>GPLGSIYSPHETLAEKHSEKKLMDSFSPSLSQDKMDGEFAHANIDGISIRLCLNKGICSVFYLDGDKIQSTQLSSKEYNNLLSSLPPKQFNLGKVHTITAPVSGNFKTHKPAPEVIETAINCCTSIIPNDDYFHVKDTDFNSVWHDIYRDIRASDSNSTKIYFNNIEIPLKLIADLINELGINEFIDSKKELQMLSYNQVNKIINSNFPQQDLCFQTEKLLFTSLFQDPAFISALTSAFWQSLHITSSSVEHIYAQIMSENIENRLNFMPEQRVINNCGHIIKINAVVPKNDTAISASGGRAYEVSSSILPSHITCNGVGINKIETSYLVHAGTLPSSE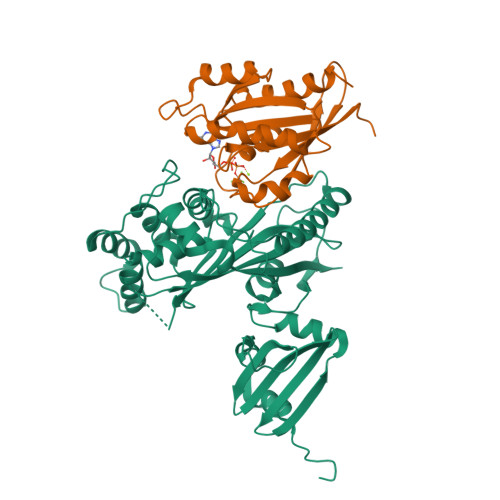GLRNAIPPESRQVSFAIISPDV[3x];>[3x]PEYDALFKLLLIGDSGVGKSCLLLRFADDTYTESYISTIGVDFKIRTIELDGKTIKLQIWDTAGQERFRTITSSYYRGAHGIIVVYDVTDQESFNNVKQWLQEIDRYASENVNKLLVGNKCDLTTKKVVDYTTAKEFADSLGIPFLETSAKNATNVEQSFMTMAAEIKKRM> MASTKSELIERLATQQSHIPAKTVEDAVKEMLEHMASTLAQGGSGGLTKAE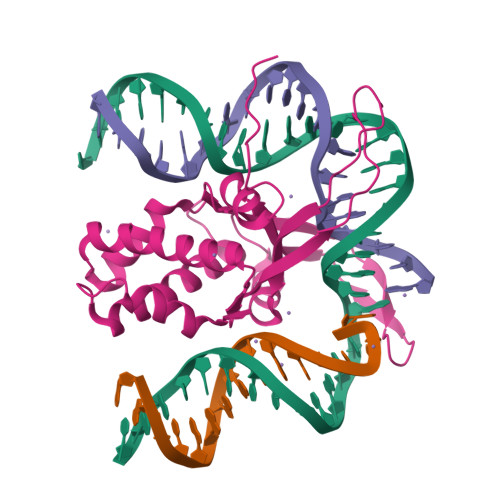MSEYLFDKLGLSKRDAKELVELFFEEIRRALENGEQVELSGFGNFDLRDKNQRPGRNPKTGEDIPITARRVVTFRPGQKLKSRVENAGGGERIEIRGFGSFSLHYRAPRTGRNPKTGDKVELEGKYVPHFKPGKELRDRANIYGGSGHHHHHH> MDYKESCPSVSIPSSDEHREKKKRFTVYKVLVSVGRSEWFVFRRYAEFDKLYNSLKKQFPAMALKIPAKRIFGDNFDPDFIKQRRAGLNEFIQNLVRYPELYNHPDVRAFLQMDSPRHQSDPSEDEDERSTSKPHSTSRNINLGPTGNPHAK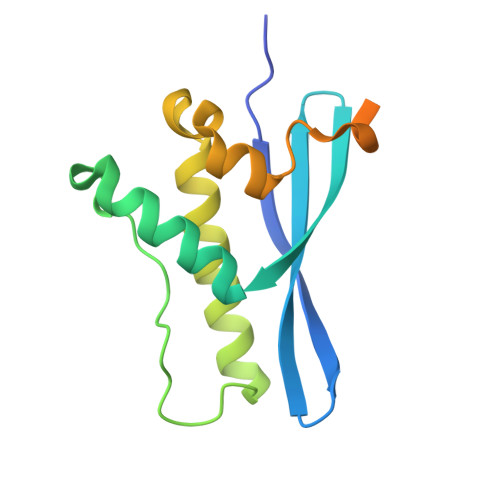PT> M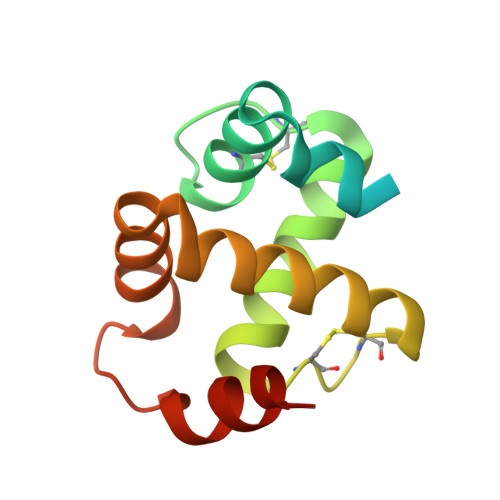NFLVLSIVVTMAAFVAAETYTDRYDHINIDEIIENRKLLVPYIKCTLDQGRCTPEGRELKAHIKDAMQTSCSKCTEKQKKGARKVVRHIRAKEQEYWKQILAKYDPEDQYKENYETFLAAED> GSGGSGKVVKFSYMWTINNFSFCREEMGEVIKSSTFSSGANDKLKWCLRVNPKGLDEESKDYLSLYLLLVSCPKSEVRAKFKFS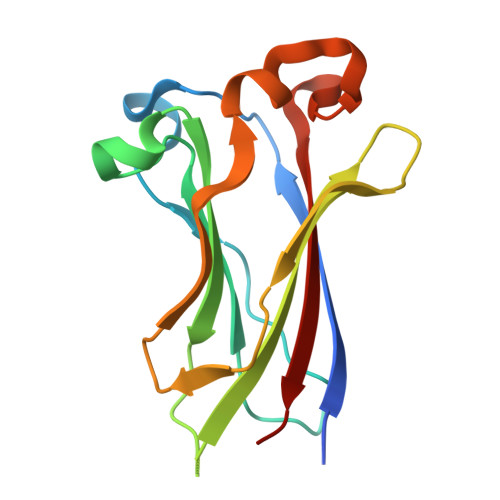ILNAKGEETKAMESQRAYRFVQGKDWGFKKFIRRDFLLDEANGLLPDDKLTLFCEVSVVQD>MAWSHPQFEKGHMNDANIADVVTKVLGEYGAPGAVSVAALTAKSPDGKSNSSADADVVARMVAKAIRDHAGTAQPSGNAATSSAAVSDGVFETMDAAVEAAALAQQQYLLCSMSDRARFVQGIRDVILNQDTLEKMSRMAVEETGMGNYEHKLIKNRLAGEKTPGIEDLTTDAFSGDNGLTLVEYSPFGVIGAITPTTNPTETIVCNSIGMLAAGNSVVFSPHPRARQVSLLLVRLINQKLAALGAPENLVVTVEKPSIENTNAMMAHPKVRMLVATGGPAIVKAVLSTGKKAIGAGAGNPPVVVDETANIEKAACDIVNGCSFDNNLPXVAEKEIIAVAQIADYLIFNLKKNGAYEIKDPAVLQQLQDLVLTAKGGPQTKCVGKSAVWLLSQIGIS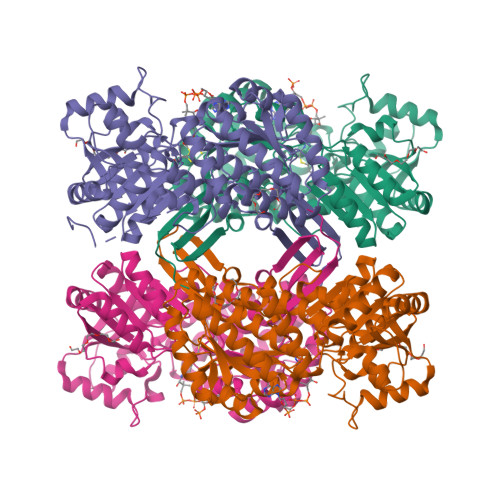VDASIKIILMEVPREHPFVQEELMMPILPLVRVETVDDAIDLAIEVEHDNRHTAIMHSTDVRKLTKMAKLIQTTIFVKNGPSYAGLGAGGEGYSTFTIAGPTGEGLTSAKSFARRRKCVMVEALNIR[4x]>GNGKLRQWLIDQIDSGKYPGLVWENEEKSIFRIPWKHAGKQDYNREEDAALFKAWALFKGKFREGIDKPDPPTWKTRLRCALNKSNDFEELVERSQLDISDPYKVYRIVPEGAKKG[4x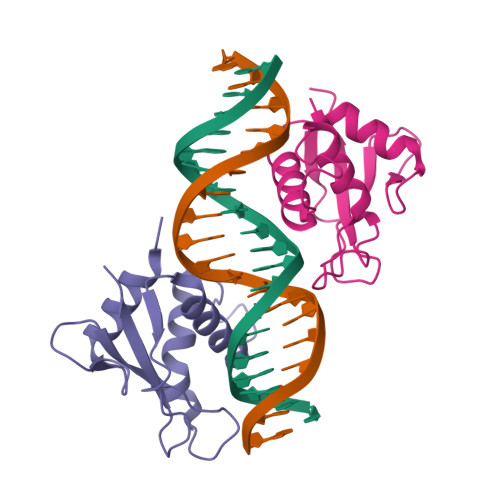]> SKMSDVKCTSVVLLSVLQQLRVESSSKLWAQCVQ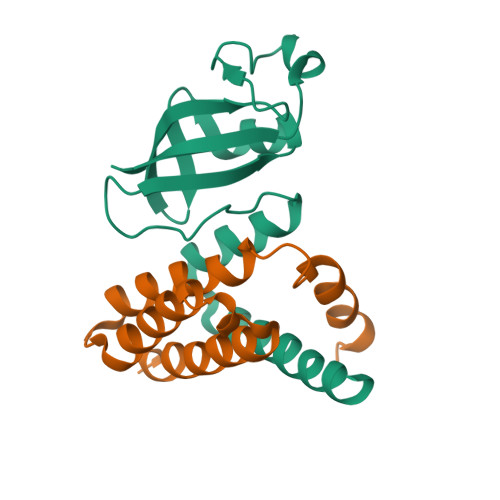LHNDILLAKDTTEAFEKMVSLLSVLLSMQGAVDINKLCEEMLDNRATL;> AIASEFSSLPSYAAFATAQEAYEQAVANGDSEVVLKKLKKSLNVAKSEFDRDAAMQRKLEKMADQAMTQMYKQARSEDKRAKVTSAMQTMLFTMLRKLDNDALNNIINNARDGCVPLNIIPLTTAAKLMVVIPDYNTYKNTCDGTTFTYASALWEIQQVVDADSKIVQLSEISMDNSPNLAWPLIVTALRANSAVKLQ> TKGLVLGIYSKEKEEDEPQFTSAGENFNKLVSGKLREILNISGPPLKAGKTRTFYGLHEDFPSVVVVGLGKKTAGIDEQENWHEGK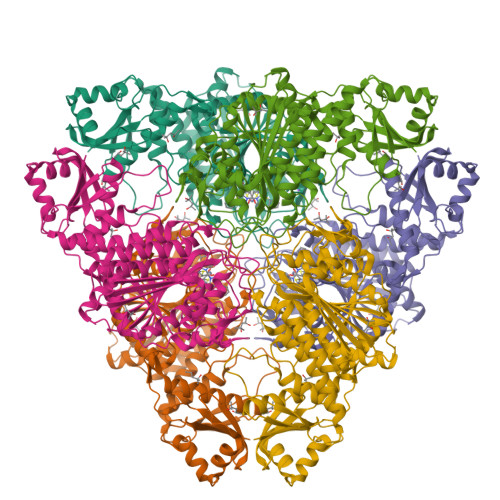ENIRAAVAAGCRQIQDLEIPSVEVDPCGDAQAAAEGAVLGLYEYDDLKQKRKVVVSAKLHGSEDQEAWQRGVLFASGQNLARRLMETPANEMTPTKFAEIVEENLKSASIKTDVFIRPKSWIEEQEMGSFLSVAKGSEEPPVFLEIHYKGSPNASEPPLVFVGKGITFDSGGISIKAAANMDLMRADMGGAATICSAIVSAAKLDLPINIVGLAPLCENMPSGKANKPGDVVRARNGKTIQVDNTDAEGRLILADALCYAHTFNPKVIINAATLTGAMDIALGSGATGVFTNSSWLWNKLFEASIETGDRVWRMPLFEHYTRQVIDCQLADVNNIGKYRSAGACTAAAFLKEFVTHPKWAHLDIAGVMTNKDEVPYLRKGMAGRPTRTLIEFLFRFSQDS> KYNKEFLLYLAGFVDGDGSIIAQIKPN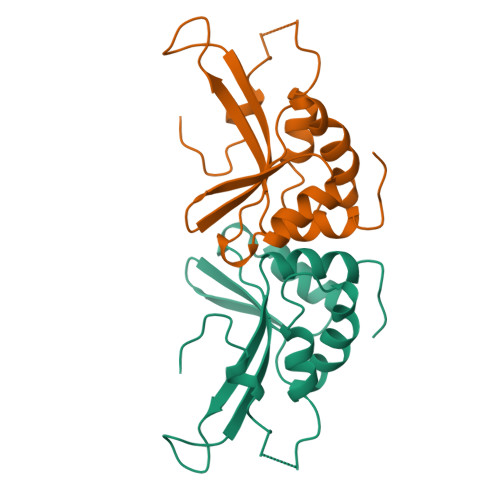QSYKFKHQLSLTFQVTQKTQRRWFLGKLVDEIGVGYVRDRGSVSDYILSEIKPLHNFLTQLQPFLKLKQKQANLVLKIIEQLPSAKESPDKFLEVCTWVDQIAALNDS> MRAVVVGAGLGGLLAGAFLARNGHEIIVLEKSAMIGGRFTNLPYKGFQLSTGALHMIPHGEDGPLAHLLRILGAKVEIVNSNPKGKILWEGKIFHYRESWKFLSVKEKAKALKLLAEIRMNKLPKEEIPADEWIKEKIGENEFLLSVLESFAGWADSVSLSDLTALELAKEIRAALRWGGPGLIRGGCKAVIDELERIIMENKGKILTRKEVVEINIEEKKVYTRDNEEYSFDVAISNVGVRETVKLIGRDYFDRDYLKQVDSIEPSEGIKFNLAVPGEPRIGNTIVFTPGLMINGFNEPSALDKSLAREGYTLIMAHMALKNGNVKKAIEKGWEELLEIFPEGEPLLAQVYRDGNPVNRTRAGLHIEWPLNEVLVVGDGYRPPGGIEVDGIALGVMKALEKLNLGSFSEWYL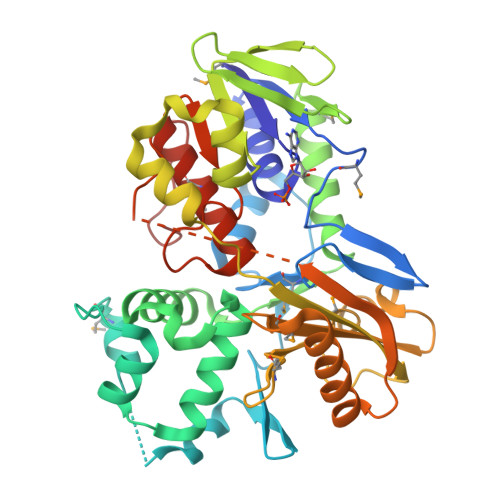LEHHHHHH{[(2R,3R,4R,5R)-3-(alpha-D-glucopyranosyloxy)-4-hydroxy-2,5-bis(hydroxymethyl)pyrrolidin-1-yl]methyl}phosphonic 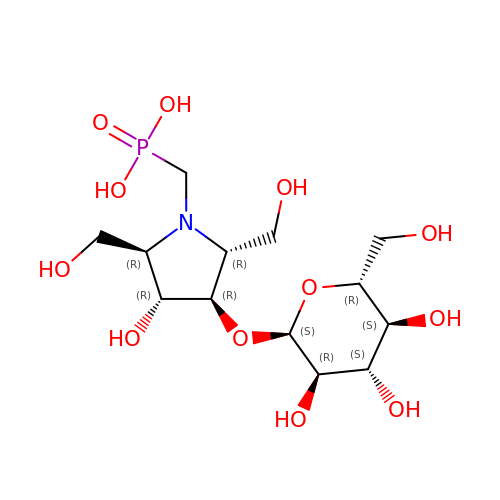acid | C13 H26 N O12 P | QVTCDBMCRXGRKE-DFIZWEOJSA-N> MQPFDSGHDDLVHDVVYDFYGRHVATCSSDQHIKVFKLDKDTSNWELSDSWRAHDSSIVAIDWASPEYGRIIASASYDKTVKLWEEDPDQEECSGRR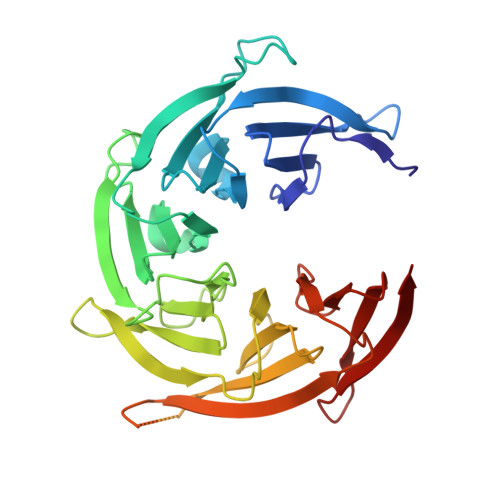WNKLCTLNDSKGSLYSVKFAPAHLGLKLACLGNDGILRLYDALEPSDLRSWTLTSEMKVLSIPPANHLQSDFCLSWCPSRFSPEKLAVSALEQAIIYQRGKDGKLHVAAKLPGHKSLIRSISWAPSIGRWYQLIATGCKDGRIRIFKITEKLSPLASEESLTNSNMFDNSADVDMDAQGRSDSNTEEKAELQSNLQVELLSEHDDHNGEVWSVSWNLTGTILSSAGDDGKVRLWKATYSNEFKCMSVIT> WMLDPIAGKWSR;> MIDKSAFVHPTAIVEEGASIGANAHIGPFCIVGPHVEIGEGTVLKSHVVVNGHTKIGRDNE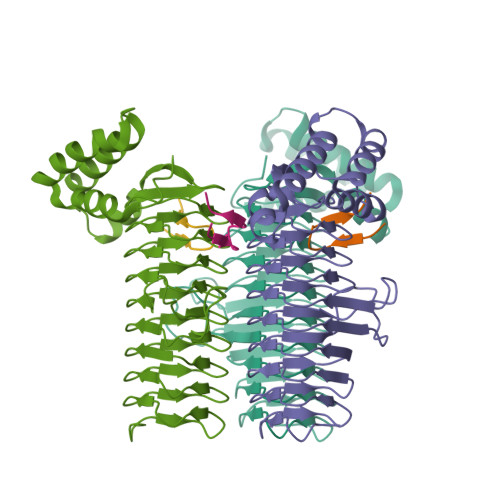IYQFASIGEVNQDLKYAGEPTRVEIGDRNRIRESVTIHRGTVQGGGLTKVGSDNLLMINAHIAHDCTVGNRCILANNATLAGHVSVDDFAIIGGMTAVHQFCIIGAHVMVGGCSGVAQDVPPYVIAQGNHATPFGVNIEGLKRRGFSREAITAIRNAYKLIYRSGKTLDEVKPEIAELAETYPEVKAFTDFFARSTRGLIR> GAMGKCPTKVVLLRNMVGA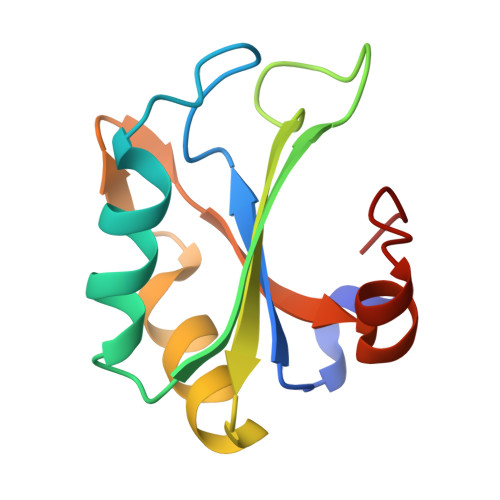GEVDEDLEVETKEECEKYGKVGKCVIFEIPGAPDDEAVRIFLEFERVESAIKAVVDLNGRYFGGRVVKACFYNLDKFRVLDLAEQV>[6x]MLYSNLINVKQKVISIREKLGDPRLKSLVFEYPAGQLFRVTPKLKVSMVP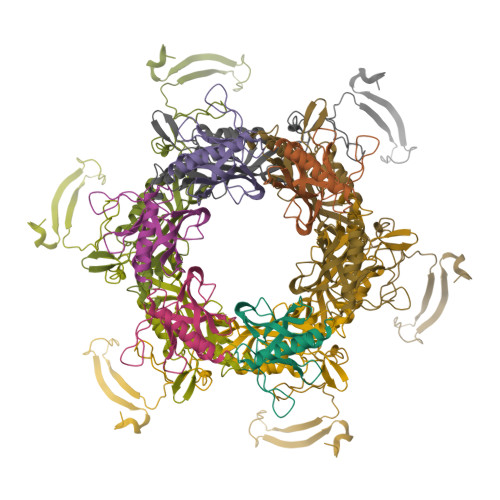KNMIGLPLDSKSNITISADDYYITDVSRNVPEAAFRTRAWLDPVINDSGVIVSGINCRCHVINDKSGLSYDLILRKEREVRV;>[6x]MTKPSLISAKILQHINSIVWLQSKGIQEPLKPDVIVNNVAYPPNVIAEKPVTNIEVITNSSMIENTGGVRQFLCKAVFEYTIVWVFSREVYKTYHQIPRSQIQDLLVFCQQFVISAYQGIDPDITNIDLKPSQVLVKPTEDVNSDVSNSSSWSVVADLRFMIEFLTSLDEFLPIDFNKIQPPTWELLDDLDPIVPEQPFTLNGLIISLNKSELPKVRADESDTYQLEEILYIPPTIEDQI> GSHMKPHPWFFGKIPR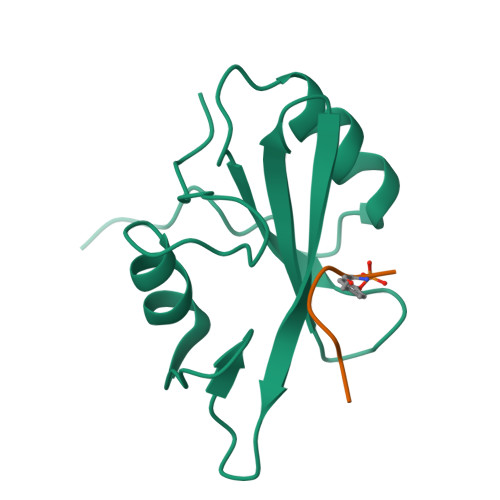AKAEEMLSKQRHDGAFLIRESESAPGDFSLSVKFGNDVQHFKVLRDGAGKYFLWVVKFNSLNELVDYHRSTSVSRNQQIFLRDIE;> QNGYENPTY>[2x]SNAMKNILSIQSHVVFGHAGNSAAEFPMRRMGVNVWPLNTVQFSNHTQYGHWTGCVMPA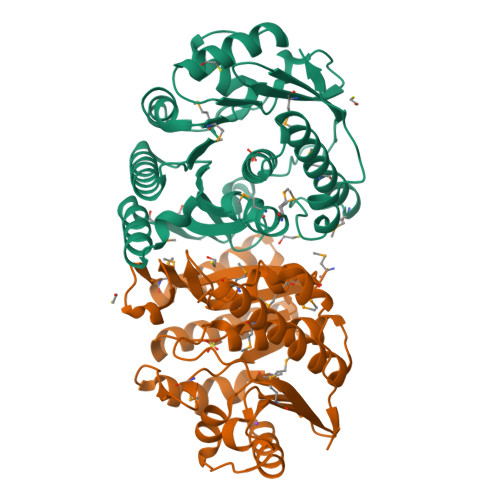SHLTDIVQGIADIDRLKDCDAVLSGYIGSPEQGSHILAAVAQVKQANPDAWYFCDPVMGHPEKGCIVAPGVAEFFCNEALPASDMIAPNLLELEQLSGERVENVEQAVQVARSLCARGPKVVLVKHLSRAGYHADCFEMLLVTADDAWHICRPLVDFGKRQPVGVGDLTSGLLLVNLLKGEPLDKALEHVTAAVYEVMLKTQEMGEYELQVVAAQETIVTPICQFTAVRL> MNSPISPIETVPVKLKPGMDGPKVKQWPLTEEKIKALVEICTEMEKEGKISKIGPENPYNTPVFAIKKKDSTKWRKLV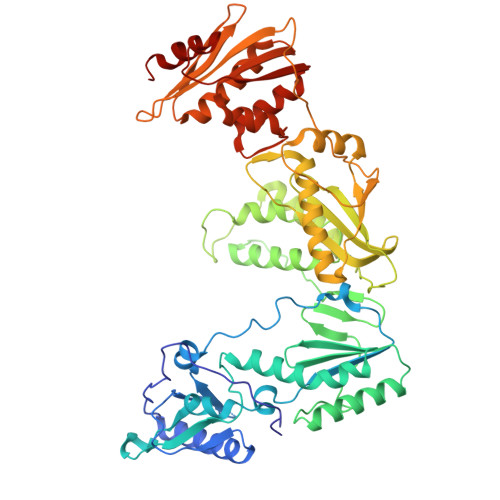DFRELNKRTQDFWEVQLGIPHPAGLKKNKSVTVLDVGDAYFSVPLDEDFRKYTAFTIPSINNETPGIRYQYNVLPQGWKGSPAIFQSSMTKILEPFRKQNPDIVIYQYMDDLYVGSDLEIGQHRTKIEELRQHLLRWGLTTPDKKHQKEPPFLWMGYELHPDKWTVQPIVLPEKDSWTVNDIQKLVGKLNWASQIYPGIKVRQLCKLLRGTKALTEVIPLTEEAELELAENREILKEPVHGVYYDPSKDLIAEIQKQGQGQWTYQIYQEPFKNLKTGKYARMRGAHTNDVKQLTEAVQKITTESIVIWGKTPKFKLPIQKETWETWWTEYWQATWIPEWEFVNTPPLVKLWYQLEKEPIVGAETFYVDGAANRETKLGKAGYVTNRGRQKVVTLTDTTNQKTELQAIYLALQDSGLEVNIVTDSQYALGIIQAQPDQSESELVNQIIEQLIKKEKVYLAWVPAHKGIGGNEQVDKLVSAGIRKVL2,4-dibromo-6-({[(2-nitrophenyl)carbonyl]amino}methyl)phenyl 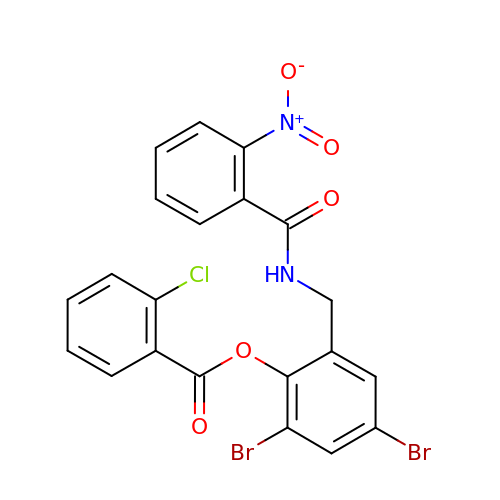2-chlorobenzoate | C21 H13 Br2 Cl N2 O5 | WKUUVOPOQKZMFY-UHFFFAOYSA-N Here, we report the atomic structures of an engineered diffocin, a contractile syringe-like molecular machine that kills the Gram-positive bacterium Clostridioides difficile. Captured in one pre-contraction and two post-contraction states, each structure fashions six proteins in the bacteria-targeting baseplate, two proteins in the energy-storing trunk, and a collar linking the sheath with the membrane-penetrating tube. Specific attachment of baseplate tail fibers to receptors on the surface of a target bacterial cell triggers conformational changes of the neighboring baseplate, which leads to reorientation of sheath proteins and contraction of the entire sheath assembly. Since the sheath and the tube are anchored together at the opposite end by the collar, collapsing the sheath pushes the tube through the baseplate, driving it to puncture the cell wall and underlying cytoplasmic membrane.

CryoEM data processing of the post-contraction diffocin particles resolved two different substates, an apparent transitional state and a final state, which is 2 nm shorter in length. The four-layer sheath near the collar only contracts partially in the transitional state, allowing for the tube to be extended an additional 2 nm in the final state. In the transitional state, these sheath layers are partially contracted, as indicated by the gradually decreasing diameter of the hexameric sheath rings from L28 to L32. Specifically, the diameter of L28 in the transitional state is similar to that in the final state, while the diameter of L32 in the transitional state is almost identical to that in the pre-contraction state. Consequently, the last few sheath layers still interact with the central tube in the transitional state. The N-terminal domain of the collar subunit binds to the tube, while its C-terminal β-strand extends towards the C-terminal β-hairpin of last sheath, forming a three-β-strand handshake interaction. The insufficient contraction of the sheath and the absence of additional collar-sheath interactions indicate that the transitional state is metastable relative to the final state and has potential for further contraction. However, contraction of the diffocin pauses at collar-proximal sheath layers prior to completion, giving rise to two post-contraction states. The observation that sheath layers on the baseplate side are fully contracted, while those on the collar side are partially contracted, supports the wave-like propagation model from the baseplate to the collar, and our structure of the diffocin in the transitional state provides atomic resolution details of a intermediate of potential relevance to other Gram-positive CISs.

>[18x]MANMEARNVMSGTWGELWLDGNKVAEVKKFQAKMEFTKEDIIIAGQMGTDTKYMGYKGKGSITLYHVSSRMHKLIGEKIKRGSEPRFVAISKLNDPDSYGAERIAVKNIAFDDLTLADWEVGVKGEIEAPFTFTEYDFLDII;>MAIGLPSINISFKELATTVKERSARGIIAMVLKDAKALGLNEIHEKEDIPVDLSAENKEYINLALMGNVNTPNKLLVYVIEGEADIQTALDFLETKEFNYLCMPKAVEADKTAIKNWIIKLRDIDKVKVKAVLGKVVGNHEGIINFTTEDVLVGEKKYSVDEFTSRVAGLIAGTPLSQSVTYTKLSDVVDIPKMTKVDAESRVNKGELILIKEAGAIRIARGVNSLTELTAEKGEMFQKIKIVDTLDIIHSDIRKVIIDDYIGKVTNSYDNKCLLIVAIKSYLEELEKSALIESDSTVEIDFEAQKSYLKSKGVDLSYMTLQEIKEANTGSKVFLKAKIKVLDAMEDIDLSIEI[18x];>[6x]MLKYKEILETIIEILKKNFTESIFIDDESVQGSEGSCFFVSILSVICTPVMLNTNNKDIVISIKYLPKPQSKSIRMYEISDELNKLFNRNIKVTDRKLNITKLEQSIKKEESIYVLNFTFTLNYLDSVYEEDVVYENMKEINLNLGE> GHLPKPTLWAEPGSVITQGSPVTLRCQGGQETQEYRLYREKKTAPWITRIPQELVKKGQFPIPSITWEHTGRYRCYYGSDTAGRSESSDPLELVVTGAYIKPTLSAQPSPVVNSGGNVTLQCDSQVAFDGFILC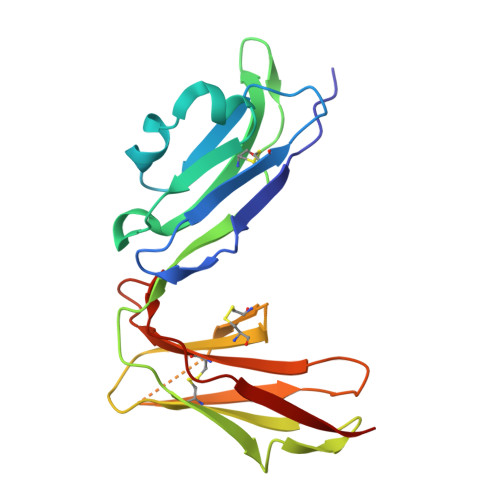KEGEDEHPQCLNSQPHARGSSRAIFSVGPVSPSRRWWYRCYAYDSNSPYEWSLPSDLLELLVLG>MIICSVDIGIKNPAYAIFNYDNTSNTIKLIAIEKSDWTKNWERSVARDLTRYNPDVVILEKQGFKSPNSKIIYFIKGFFYNSNTKVIVRNPTFKGGSYRNRKKQSIDVFIQKISEYTDYKNDILNKYTKLDDIANSFNLGLSYMESLLK[4x]

The DNA resolvases orthologous to the A22 protein of vaccinia virus play an essential role in poxviral replication, by resolving HJ structures formed at the inverted repeat junctions in a concatemer of linear genomic DNAs. The poxvirus resolvases belong to the RNaseH/retroviral integrase superfamily of DNA-modifying enzymes that employ a conserved metal-dependent mechanism, including the prototypical bacterial RuvC HJ DNA resolvase. The fowlpox virus resolvase (Fpr) forms a stable dimer as other homologous resolvases14–17 and was found to bind to various structural motifs on the HJ DNA, revealing flexibility of the Fpr dimer in binding to a wide range of DNA structures. The 150-residue Fpr protein has the characteristic architecture of enzymes from the retrovirus integrase/RNase H superfamily, comprising a single layer of β-sheet sandwiched between α-helices.

Eventually, the Holliday junction HJ8/5, which has two 5 bp arms covalently closed with -TTT- hairpins and 8 bp arms with blunt ends, gave crystals that diffracted to ~3.3 Å resolution. Unexpectedly, the crystal structure of the Fpr-HJ8/5 complex reveals that the HJ is in a H-stacked conformation, where arms 1 and 4 (as well as arms 2 and 3) of HJ8/5 stack on each other to form a pseudo-continuous double-helix. The two pseudo-continuous helices are linked by a crossover of backbones and are arranged in an antiparallel orientation with an angle between their axes of ~30°. In the Fpr-HJ8/5 complex crystal lattice, an asymmetric unit contains one DNA Holliday junction and two copies of Fpr dimers (4:1 Fpr monomer: HJ ratio). Each HJ is surrounded by a total of 4 Fpr dimers (including two symmetry-related dimers). The Fpr dimers make extensive contacts and bridges between HJ-DNA molecules. These interactions are formed with various structural motifs from different regions of the HJ-DNA: TTT hairpin-loop, the crossover junction, and double-stranded DNA. The -TTT- hairpin-loop fits into a positively charged groove at the dimer interface formed between αA/αB and αB/β5 of the two monomers. This interaction includes DNA backbone contacts by Trp41, Pro67, Lys70, and Tyr73, as well as electrostatic and van der Waals contacts with a flipped-out thymine base by Phe64, Ser69, and Ile72. At the center of HJ-DNA, the N-terminus of the αC helix and the preceding loop (between β5 and αC) contact the crossover junction, with a stretch of residues Ser97-Tyr98-Arg99 at the apex positioned over the DNA minor groove. DNA strands near the stacked blunt ends are bound in the basic groove across the Fpr dimer interface, similarly to the -TTT- hairpin-loop but on the opposite side of the Fpr dimer.>SNAMAAKKPLFEVIASKIKDSINRDEYKTGMLMPNETALQEIYSSSRTTIRR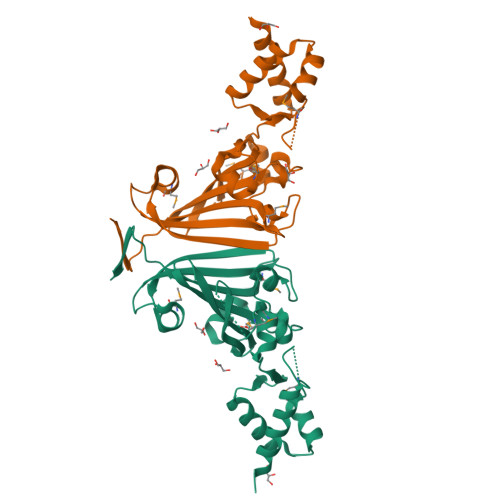AVDLLVEEGLVVRKNGVGLYVQPKLTAQNILEMTGVMKNDTNENLKKDIKDFYIRKAGKFYAEIFGMKENELVYSIKFVQKSEHGATLDRLILPLGLYPDLQAKDFQIINIIELVNSGKYKLFELEQELQLILAGNEQIKNMHLNENDPVFKLSSVFYAENDMPIAIQYHYEDAESTKYVVDFN[2x]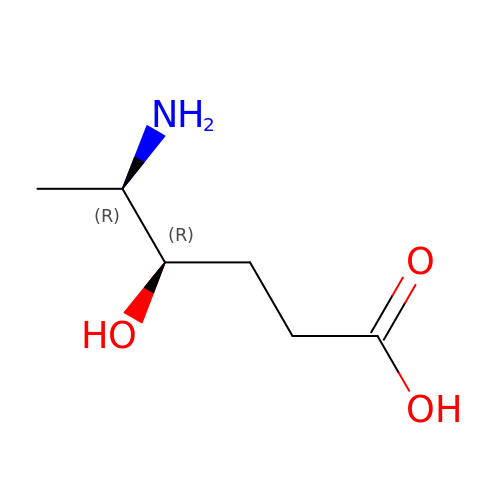5-AMINO-4-HYDROXYHEXANOIC ACID | C6 H13 N O3 | LUMVYMITQCJEGS-RFZPGFLSSA-N> GSTVTVPIAVGESDFENLNTEGSLVPRGSKSDSNASFLRAARAGNLDKVVEYLKGGIDINTCNQNGLNALHLAAKEGHVGLVQELLGRGSSVDSATKKGNTALHIASLAGQAEVV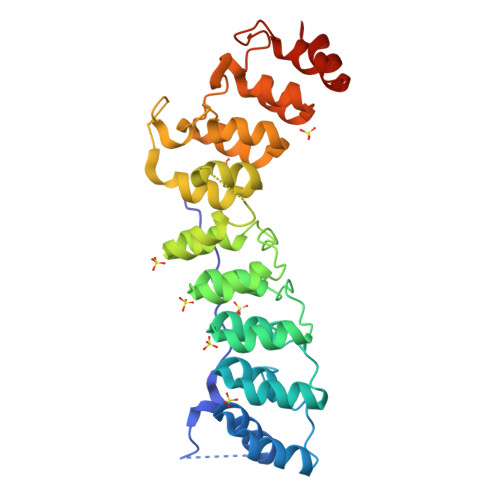KVLVKEGANINAQSQNGFTPLYMAAQENHIDVVKYLLENGANQSTATEDGFTPLAVALQQGHNQAVAILLENDTKGKVRLPALHIAARKDDTKSAALLLQNDHNADVQSKMMVNRTTESGFTPLHIAAHYGNVNVATLLLNRGAAVDFTARNGITPLHVASKRGNTNMVKLLLDRGGQIDAKTRDGLTPLHCAARSGHDQVVELLKVVTEEVTT>[2x]XEVE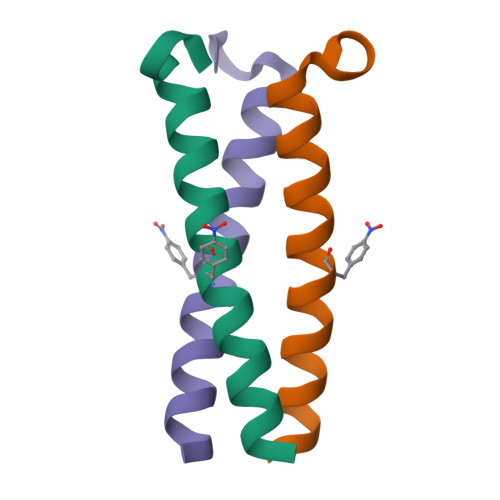ALEKKVEALEFKVQKLEKKVEALEHGWDGR> MREESTDECDGAIIGTAVKGHVAVHSDLSY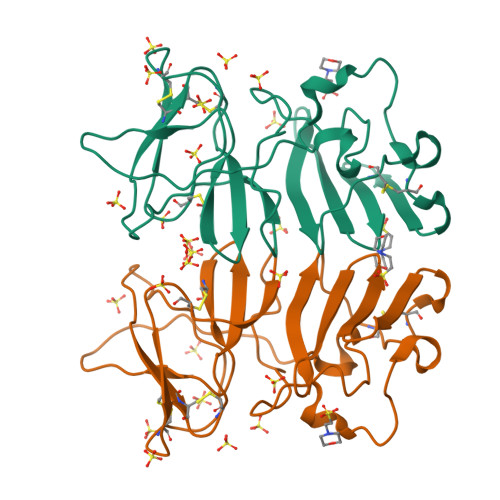WIESRYNDTWKLERAVFGEVKSCTWPETHTLWGDDVEESELIIPHTIAGPKSKHNRREGYKTQNQGPWDENGIVLDFDYCPGTKVTITEDCSKRGPSVRTTTDSGKLITDWCCRSCSLPPLRFRTENGCWYGMEIRPVMHDETTLVRSQVDA(3alpha,5alpha,8alpha)-17-(pyridin-3-yl)androst-16-en-3-ol | C24 H33 N O | 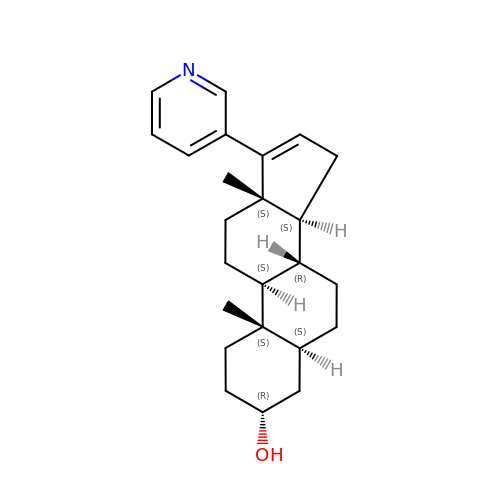UNJQRCXVHBZVTM-PFQGPGDOSA-N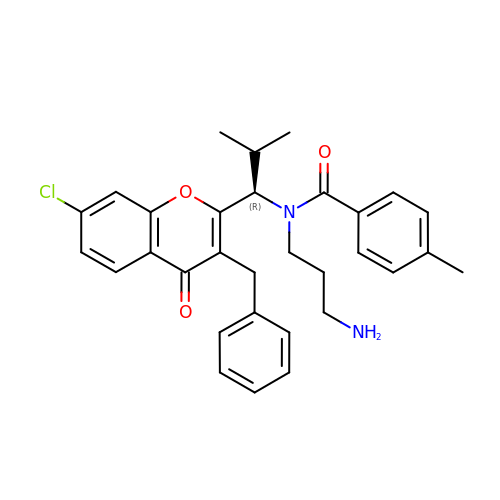N-(3-aminopropyl)-N-[(1R)-1-(3-benzyl-7-chloro-4-oxo-4H-chromen-2-yl)-2-methylpropyl]-4-methylbenzamide | C31 H33 Cl N2 O3 | PGXYIBJJCLWJST-MUUNZHRXSA-N> SSRKLTDISACSINIFYSTLGGSTQKFAEHVADRIRSSLQTELVEILNLDYIDLDEYFSKGNSNTVYLVLLPSYAIESSIDYFLSALQTTIDDFRIVARPLEKLRGFAVLGFGDFEQYAGDLFCYQAIAADQRLAKLGAQRIAPLGVVNVKLEKAQVYEAMEAWTDLFLQYAKEKA

The S-adenosyl-L-methionine-dependent tRNA 4-demethylwyosine synthase TYW1 catalyzes biosynthesis of 4-demethylwyosine (imG-14), the precursor for wyosine, the hypermodified guanine-derived nucleotide present at position 37 of phenylalanine tRNAs of archaea and eukarya. Eukaryotic TYW1 enzymes contain N-terminal flavodoxin-like and C-terminal radical-SAM domains.

We determined co-crystal structures of the flavodoxin-like domain of the putative Tyw1 from Schizosaccharomyces japonicus in complex with flavin mononucleotide (FMN), exploiting an unexpected anomalous scatterer present in the recombinant protein. Our results show how eukaryotic TYW1 enzymes bind the coenzyme FMN and will help further elucidation of the structural enzymology of 4-demethylwyosine synthesis.> MGSQVSTQRSGSHENSNSATEGSTINYTTINYYKDSYAATAGKQSLKQDPDKFANPVKDVFTEMAAPLKSPSAEACGYSDRVAQLTIGNSTITTQAAANIIVGYGEWPSYCSDDDATAVDKPTRPDVSVNRFYTLDTKLWEKSSK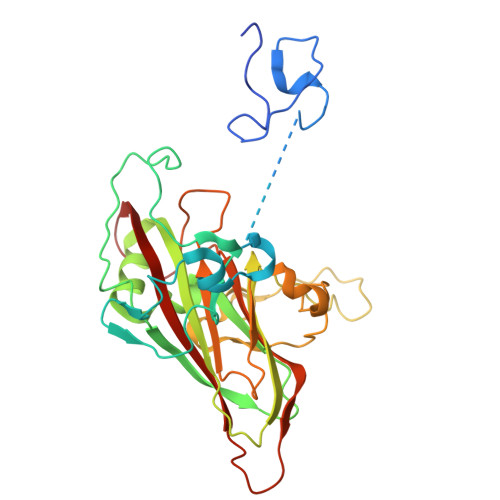GWYWKFPDVLTETGVFGQNAQFHYLYRSGFCIHVQCNASKFHQGALLVAILPEYVIGTVAGGTGTEDSHPPYIQTQPGADGFELQHPYVLDAGIPISQLTVCPHQWINLRTNNCATIIVPYMNTLPFDSALNHCNFGLLVVPISPLDFDQGATPVIPITITLAPMCSEFAGLRQAVTQ> MNTPEHMTAVVQRYVAALNAGDLDGIVALFADDATVEEGGGGEPRSGT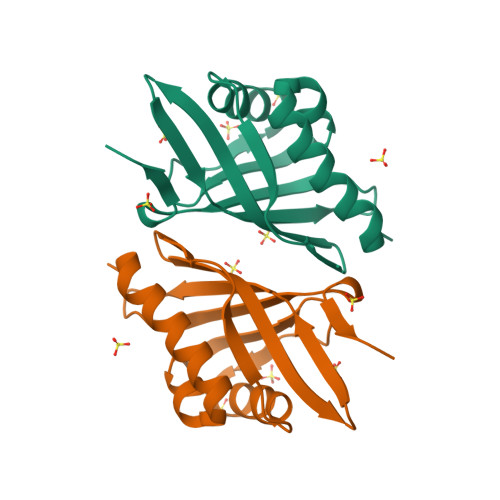AAIREFYANSLKLPLAVELTQEVRAVANEAAFAFTVSFEYQGRKTVVAPIDHFRFNGAGKVVSMRALFGEKNIHAGA> MPVFDEPVYTVNVLENSPINTLVIDLNATDPDEGTNGEVVYSFINFVSNLTKQMFKIDPKTGVITVNGVLDHEELHIHEIDVQAKDLGPNSIPAHCKVIVNVIDINDNAPEIKLLSENSEMVEVSENAPLGYVIALVRVSDNDSGANGKVQCRLQGNVPFRLNEFESFSTLLVDGRLDREQRDMYNLTILAEDSGYPPLRSSKSFAVKVTDENDNPPYFTKPHYQAMVLENNVPGAFLLAVSARDPDLGMNGTVSYEIIKSEVRGMSVESYVTVNSNGEIYGVRAFNHEDTRTFEFKVSAKDGGDPPLTSNATVRIVVLDVNDNTPVMTTPPLVNGTAEVSIPKNAGVGYLVTQIKADDYDEGENGRLTYSISEGDMAYFEIDQINGEVRTTKTFGENAKPSYQITVVAHDHGQTSLSASAYIVIYLSPDLNAQEL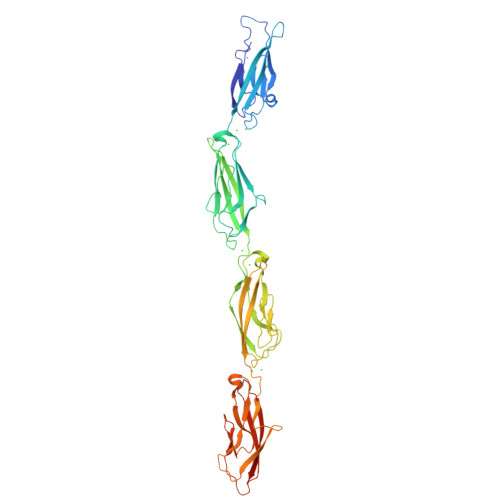EHHHHHH>[2x]MQKR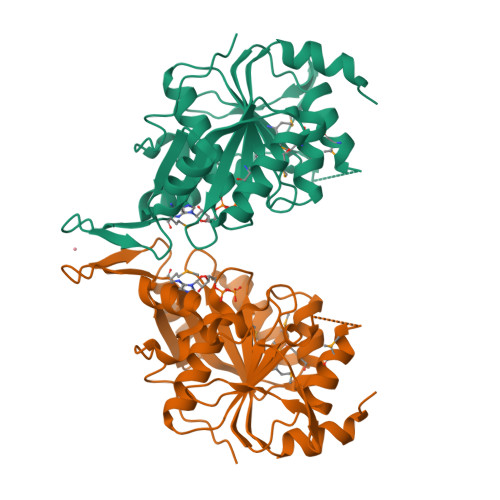VTDEDIKERLDKIGFRIAVMSGKGGVGKSTVTALLAVHYAKQGKKVGILDADFLGPSIPHLFGLEKGKVAVSDEGLEPVLTQRLGIKVMSIQFLLPKRETPVIWRGPLIAGMIREFLGRVAWGELDYLLIDLPPGTGDAPLTVMQDAKPNGAVIVSTPQELTAAVVEKAITMAEQTKTAVLGIVENMAYFECPNCGERTYLFGEGKASELARKYKIEFITEIPIDSDLLKLSDLGRVEEYEPDWFEFFPYLEHHHHHH> MASNEGVENRPFPYLTVDADLLSNLRQSAAEGLFHSFDLLVGKDAREAGIKFEVLLGVYTNAIQYVRFLETALAVSCVNTEFKDLSRMTDGKIQFRISVPTIAHGDGRRPSKQRTFIVVKNCHKHHISTEMELSMLDLEILHSIPETPVEYAEYVGAVKTVASALQFGVDALERGLINTVLSVKLRHAPPMFILQTLADPTFTERGFSKTVKSDLIAMFKRHLLEHSFFLDRAENMGSGFSQYVRSRLSEMVAAVSGESVLKGVSTYTTAKGGEPVGGVFIVTDNVLRQLLTFLGEEADNQIMGPSSYASFVVRGENLVTAVSYGRVMRTFEHFMARIVDSPEKAGSTKSDLPAVAAGVEDQPRVPISAAVIKLGNHAVAVESLQKMYNDTQSPYPLNRRMQYSYYFPVGLFMPNPKYTTSAAIKMLDNPTQQLPVEAWIVNKNNLLLAFNLQNALKVLCHPRLHTPAHTLNSLNAAPAPRDRRETYSLQHRRPNHMNVLVIVDEFYDNKYAAPVTDIALKCGLPTEDFLHPSNYDLLRLELHPLYDIYIGRDAGERARHRAVHRLMVGNLPTPLAPAAFQEARGQQFETATSLAHVVDQAVIETVQDTAYDTAYPAFFYVVEAMIHGFEEKFVMNVPLVSLCINTYWERSGRLAFVNSFSMIKFICRHLGNNAISKEAYSMYRKIYGELIALEQALMRLAGSDVVGDESVGQYVCALLDPNLLPPVAYTDIFTHLLTVSDRAPQIIIGNEVYADTLAAPQFIERVGNMDEMAAQFVALYGYRVNGDHDHDFRLHLGPYVDEGHADVLEKIFYYVFLPTCTNAHMCGLGVDFQHVAQTLAYNGPAFSHHFTRDEDILDNLENGTLRDLLEISDLRPTVGMIRDLSASFMTCPTFTRAVRVSVDNDVTQQLAPNPADKRTEQTVLVNGLVAFAFSERTRAVTQCLFHAIPFHMFYGDPRVAATMHQDVATFVMRNPQQRAVEAFNRPEQLFAEYREWHRSPMGKYAAECLPSLVSISGMTAMHIKMSPMAYIAQAKLKIHPGVAMTVVRTDEILSENILFSSRASTSMFIGTPNVSRREARVDAVTFEVHHEMASIDTGLSYSSTMTPARVAAITTDMGIHTQDFFSVFPAEAFGNQQVNDYIKAKVGAQRNGTLLRDPRTYLAGMTNVNGAPGLCHGQQATCEIIVT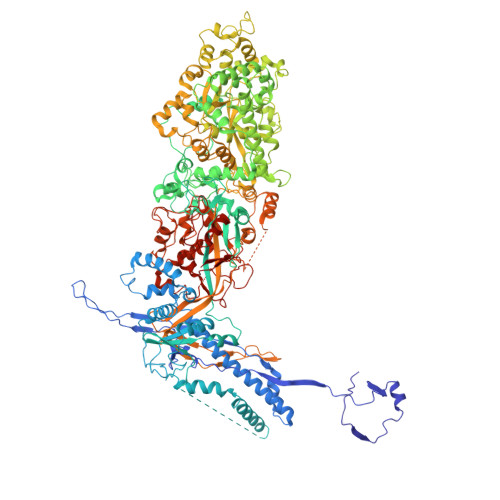PVTADVAYFQKSNSPRGRAACVVSCENYNQEVAEGLIYDHSRPDAAYEYRSTVNPWASQLGSLGDIMYNSSYRQTAVPGLYSPCRAFFNKEELLRNNRGLYNMVNEYSQRLGGHPATSNTEVQFVVIAGTDVFLEQPCSFLQEAFPALSASSRALIDEFMSVKQTHAPIHYGHYIIEEVAPVRRILKFGNKVVF(1~{S},2~{S})-~{N}'-ethanoyl-2-(3-methylphenyl)cyclopropane-1-carbohydrazide | C13 H16 N2 O2 | 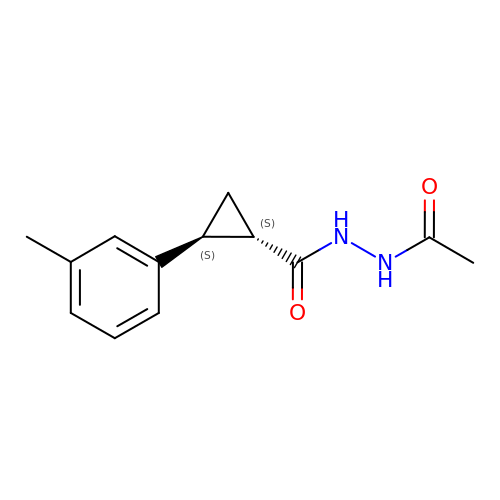ZZBMEPNWKSBENV-NEPJUHHUSA-N>[4x]MIWKRHLTLDELNATSDNTMVAHLGIVYTRLGDDVLEAEMPVDTRTHQPFGLLHGGASAALAETLGSMAG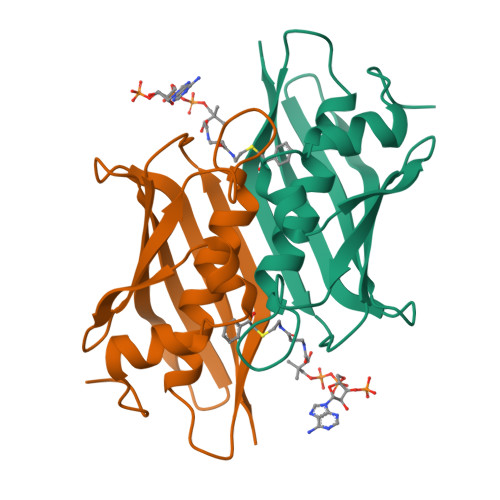FMMTRDGQCVVGTELNATHHRPVSEGKVRGVCQPLHLGRQNQSWEIVVFDEQGRRCCTCRLGTAVLG>GPLGSSYSMEQVEGITSEYIVKNADMFAVAVSLVSGKILYISNQVASIFHCKKDAFSDAKFVEFLAPHDVSVFHSYTTPYKLPPWSVCSGLDSFTQECMEEKSFFCRVSVGKHHENEIRYQPFRMTPYLVKVQEQQGAESQLCCLLLAERVHSGYEAPRIPPEKRIFTTTHTPNCLFQAVDERAVPLLGYLPQDLIETPVLVQLHPSDRPLMLAIHKKILQAGGQPFDYSPIRFRTRNGEYITLDTSWSSFINPWSRKISFIIGRHKVRVGPLNEDVFAAPPCPEEKTPHPSVQELTEQIHRLLMQPVP[2x]

PERIOD proteins are central components of the Drosophila and mammalian circadian clocks. A structural feature shared by many eukaryotic clock proteins are the PER-ARNT-SIM (PAS) domains, which represent a diverse and ubiquitous family of sensory-, signalling-, and protein-protein interaction modules. Examples include the Drosophila (d) and mouse (m) PERIOD proteins as well as the bHLH-PAS transcription factors d/mCLOCK, dCYCLE, and mBMAL1, which contain two tandemly organized PAS domains (referred to as PAS-A and PAS-B) for protein-protein interactions. Whereas the PAS domains of dPER are involved in dTIM binding, the PAS domains of mPER1, 2, and 3 mediate homo- and heterodimerization of the three PERIOD homologues in the mammalian circadian clock.

To provide insights into the PAS domain interactions of PERIOD proteins in the mammalian circadian clock, we have determined the crystal structure of the mouse PERIOD2 fragment mPER2[170–473], which includes the two PAS domains (PAS-A and PAS-B), the αE helix, and a short extension N-terminal to the PAS-A domain. The mPER2[170–473] structure was solved by molecular replacement using the refined dPER[232–599] structure as search model. The structure revealed a noncrystallographic dimer, which, in contrast to dPER, is mainly stabilized by interactions between the PAS-B β-sheet surfaces that pack against each other in an antiparallel orientation. Interestingly, the PAS-B dimer interface includes the conserved Trp419 (corresponding to Trp482 of dPER) of both monomers as a crucial interface residue. In the homodimer, both Trp419 residues are 80% buried because of stacking interactions with the preceding Pro418 as well as van der Waals interactions with Ile427, Arg429, Pro390, and Ser413 of the dimerising molecule. Overall, the PAS-B dimer interface is predominantly hydrophobic and also includes two centrally located phenylalanines, Phe415 and Phe425, which establish stacking interactions to their noncrystallographic symmetry mates. In addition to the PAS-B β-sheet interactions, the mPER2 homodimer is stabilized by interactions of the PAS-A domain with helix αE and the PAS-B domain. In molecule 1, the PAS-A β-sheet surface is covered by an intramolecular interaction with residues 170–182 located N-terminal to the PAS-A domain. Notably, the αE helix of mPER2 contains a nuclear export signal (NES) comprising residues Leu460, Ile464, Leu467, and Met469. In contrast, the single mutations of Trp419, Ile427, or Phe415 in the PAS-B dimer interface of mPER2 to Glu disrupted mPER2 homodimers under gel filtration conditions.> MALDKSIVVNLTSRLFADELAALQSKIGSVLPLGDCHRLQNIQALGLGCVCSRETSPDYIQIMQYLSKCTLAVLEEVRPDSLRLTRMDPSDNLQIKNVYAPFFQWDSNTQLAVLPPLFSRKDSTIVLESNGFDIVFPMVVPQQLGHAILQQLLVYHIYSKISAGAPGDVNMAELDLYTTNVSFMGRTYRLDVDNTDPRTALRVLDDLSMYLCILSALVP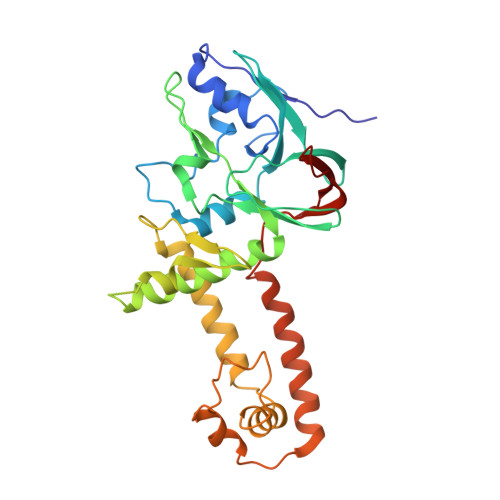RGCLRLLTALVRHDRHPLTEVFEGVVPDEVTRIDLDQLSVPDDITRMRVMFSYLQSLSSIFNLGPRLHVYAYSAETLAASCWYSPR>[2x]MEYIIKNGFVYCPLNGVDGEKMDICVKDGKIVESVSDSAKVIDASGKIVMPGGVDPHSHIAGAKVNVGRMYRPEDSKRDAEKFKGGRAGSGFSVPSTFMTGYRYAQMGYTTAMEAAMPPLLARHTHEEFHDTPIIDHAAYPLFGNNWFVMEYLKEGDVDACAAYASWLLRATKGYTIKIVNPAGTEAWGWGGNVHGIYDPAPYFDITPAEIIKGLAEVNEKLQLPHSIHL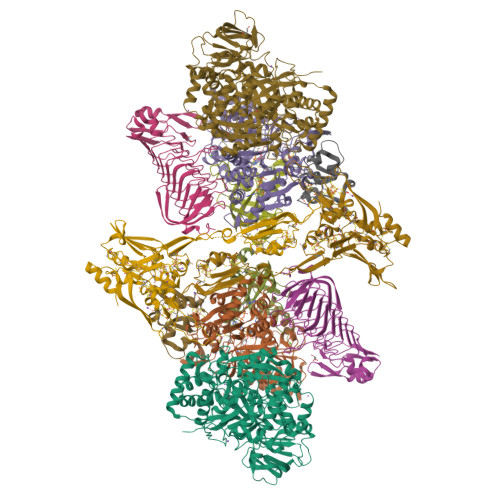HCNDLGHPGNYETTLASFDVPKNIKPNPATGSRDTVLYATHVQFHSYGGTTWRDFVSEAPKIADYVNKNDHIVIDVGQITLDETTTMTADGPMEYDLHSLNGLKWANCDVELETGSGVVPFIYSARAPVPAVQWAIGMELFLLIDNPEKVCLTTDSPNAGPFTRYPRVIAWLMSNKYRMNLIEGELHKWAQRKSTVATIDREYTFSEIAQITRATSAKVLGLSDTKGHLGVGADADIAVYDINPETVDPSAEYMAIEEAFSRAACVLKDGEIVVKDGEVVASPHGRTYWVDTQVDESIYSEVLANVESKFKQYYSVNFANYPVQDDYLPKSAPVKGVML;>[2x]MEYVKNVVCPFCGTLCDDIICKVEGNEIVGTINACRIGHSKFVHAEGAMRYKKPLIRKNGEFVEVSYDEAIDKAAKILAESKRPLMYGWSCTECEAQAVGVELAEEAGAVIDNTASVCHGPSVLALQDVGYPICTFGEVKNRADVVVYWGCNPMHAHPRHMSRNVFARGFFRERGRSDRTLIVVDPRKTDSAKLADIHLQLDFDRDYELLDAMRACLLGHEILYDEVAGVPREQIEEAVEVLKNAQFGILFFGMGITHSRGKHRNIDTAIMMVQDLNDYAKWTLIPMRGHYNVTGFNQVCTWESGYPYCVDFSGGEPRYNPGETGANDLLQNREADAMMVIASDPGAHFPQRALERMAEIPVIAIEPHRTPTTEMADIIIPPAIVGMEAEGTAYRMEGVPIRMKKVVDSDLLSDREILERLLEKVREYKASK;>MSEIILTPKEQPEVPLEAPNIKPDVFAGKSIEEIKNIQIMHGNEVVKLGDFFEVSGEPADAPEDIKIIIDGDVYNTKRIGQEMTAGEIIVRGNVNMYVGAGMKGGKITVEGNAGSWAGQDMRGGEIEILGDAGDYVGSSYRGDWRGMSGGTITVHGNADNEIGEYMNGGKIIIKGDVNIMPGIHMNNGLIIIEGNVVARAGGEMAGGTIVVKGMMQEFLAGFKYLGVEKDIEVDGEELPGAFYKFEGDHAIKGAKGIVYAAVGCNGHIAP[2x];>MRVILNTGRTIWQGQAIESGKDLKMYVDAAAIIQMNPEMMKQLGIAEGDNVKVISEYGDVVVKAVEAKEPLPEGMVYIPMGPWANRVIRPYTDSTATPSFKNIPVEIIPTDEEVLDMPTLMKVYGKVGQI[2x];>[2x]METTEVIEGKNITVERTGEENRRLIFQDCLCAVCGLCGEICPVSAIEVNPTGAMVRTEQEKSKIAIDENKCVLCGMCSSICPFQALDLQIDGTSIKELAEYPKIIKSAEIDDETCIQCKACETACPQDAITITRELPERKDLVTGEIEIDKDTCIYCGMCEEMCPVDAIEIDHQTPSSASPVVATDIRVDEDKCVHCGICKRICPVDAIMQVCRICPYGEYEIKTPEVTGTSYIDPELCVNCGWCQEICPVDAATVTKPFEGELIIDQDTCQACETCVMVCPCNVLSFPKPEKPGEKTTKLHKDERFCIYCGACERSCPVTAITVKRNRINTTPIRSKAWKNAFDSLLK;>MAIGLKAYPELCHGCGNCVIACPVNALRSPEVAGGKGPTDDVEIIMIVEDGVVNIKNPDLCGKCGTCVESCPVDAIRLEELE[2x]>[6x]MKKFVVGLSSLVLATSSFAGGGWSYHGEHGPEHWGDLKDEYIMCKIGKNQSPVDINRIVDAKLKPIKIEYRAGATKVLNNGHTIKVSYEPGSYIVVDGIKFELKQ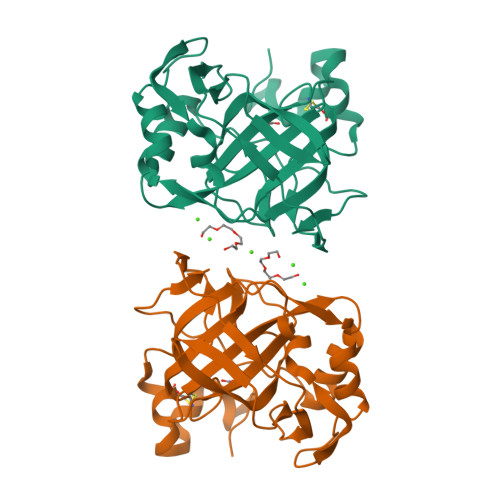FHFHAPSEHKLKGQHYPFEAHFVHADKHGNLAVIGVFFKEGRENPILEKIWKVMPENAGEEVKLAHKINAEDLLPKDRDYYRYSGSLTTPPCSEGVRWIVMEEEMEMSKEQIEKFRKIMGGDTNRPVQPLNARMIMEK>MLSRNATFNSHGQDSSYFLGWQEYEKNPYHEVHNTNGIIQMGLAENQLCFDLLESWLAKNPEAAAFKKNGESIFAELALFQDYHGLPAFKKAMVDFMAEIRGNKVTFDPNHLVLTAGATSANETFIFCLADP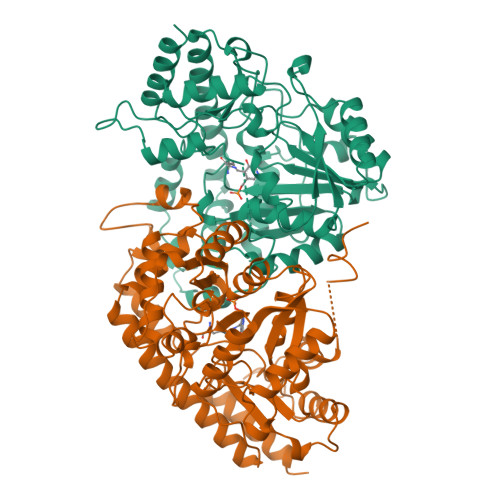GEAVLIPTPYYPGFDRDLKWRTGVEIVPIHCTSSNGFQITETALEEAYQEAEKRNLRVKGVLVTNPSNPLGTTMTRNELYLLLSFVEDKGIHLISDEIYSGTAFSSPSFISVMEVLKDRNCDENSEVWQRVHVVYSLSKDLGLPGFRVGAIYSNDDMVVAAATKMSSFGLVSSQTQHLLSAMLSDKKLTKNYIAENHKRLKQRQKKLVSGLQKSGISCLNGNAGLFCWVDMRHLLRSNTFEAEMELWKKIVYEVHLNISPGSSCHCTEPGWFRVCFANLPERTLDLAMQRLKAFVGE[2x]>[2x]MSLGDRFYDLISALHKSVRGSAPDAALYWYARILTAGGDPLYVARRLLAIASEDVGNADPRAMQVALAAW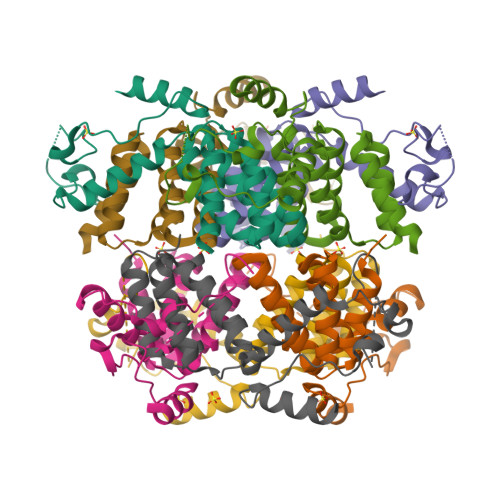DCFTRVGAYEGERAIAQAIIYLSVAPKSNAVYTAFNTAKQQAKDLPDYDVPPHLRNAPTNLMKELGYGAEYRYAHDEPNAYAAGENYFPPELKDTQYYFPTNRGMEIQIKEKLERLREQDKSTEGHHHHHH>[2x]GGUUAAAGCCUUAUGGUCGCUACCAUUGCACUCCGGUAGCGUUAAAAGGGAAGACGGGUGAGAAUCCCGCGCAGCCCCCGCUACUGUG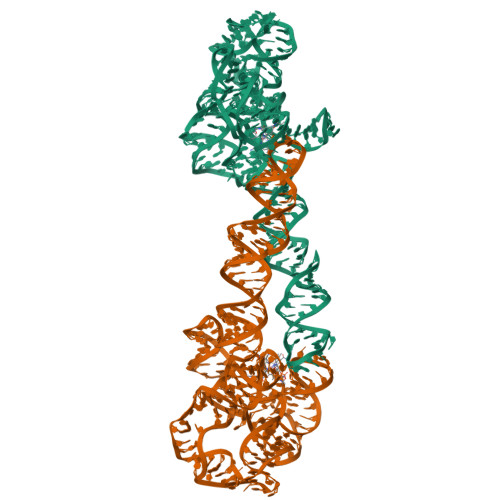AGGGAGGACGAAGCCCUAGUAAGCCACUGCCGAAAGGUGGGAAGGCAGGGUGGAGGAUGAGUCCCGAGCCAGGAGACCUGCCAUAAGGUUUUAGAAGUUCGCCUUCGGGGGGAAGGUGAACA>[2x]LDNGLARTPTMGWLHWERFMCNLDCQEEPDSCISEKLFMEMAELMVSEGWKDAGYEYLCIDDCWMAPQRDSEGRLQADPQRFPHGIRQLANYVHSKGLKLGIYADVGNKTCAGFPGSFGYYDIDAQTFADWGVDLLKFAGCYCDSLENLADGYKHMSLALNRTGRSIVYSCEWPLYMWPFQK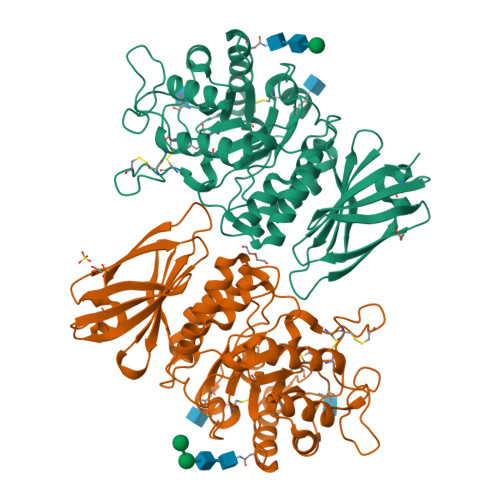PNYTEIRQYCNHWRNFADIDDSWKSIKSILDWTSFNQERIVDVAGPGGWNDPDMLVIGNFGLSWNQQVTQMALWAIMAAPLFMSNDLRHISPQAKALLQDKDVIAINQDPLGKQGYQLRQGDNFEVWERPLSGLAWAVAMINRQEIGGPRSYTIAVASLGKGVACNPACFITQLLPVKRKLGFYEWTSRLRSHINPTGTVLLQLENTMQMSLKDLLHHHHHH> YAGNPFEGVQLWANNYYRSEVHTLAIPQITDPALRAAASAVAEVPSFQWLDRNVTVDTLLVQTLSEIREANQAGANPQYAAQIVVYDLPDRDCAAAASNGEWAIANNGVNNYKAYINRIREILISFSDVRTILVIEPDSLANMVTNMNVPKCSGAASTYRELTIYALKQLDLPHVAMYMDAGHAGWLGWPANIQPAAELFAKIYEDAGKPRAVRGLATNVANYNAWSVSSPPPYTSPNPNYDEKHYIEAFRPLLEARGFPAQFIVDQGRSGKQPTGQKEWGHWCNAIGTGFGMRPTANT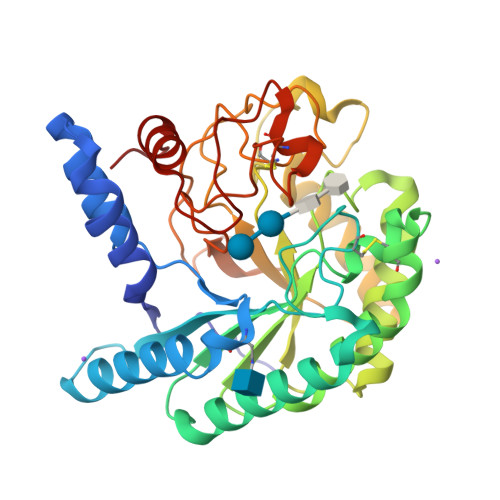GHQYVDAFVWVKPGGECDGTSDTTAARYAYHCGLEDALKPAPEAGQWFNEYFIQLLRNANPPF>[8x]MHHHHHHGENLYFQGSMLTIVQEALTFDDVLLLPAYSTVLPKDVSLKTRLTRGIYLNIPLVSAAMDTVTESRMAIAMAQNGGIGILHKNMDIAAQAAEVRRVKKFEAGKAESYPNSCKDDLGRLRVGAAVGTGADTPSRV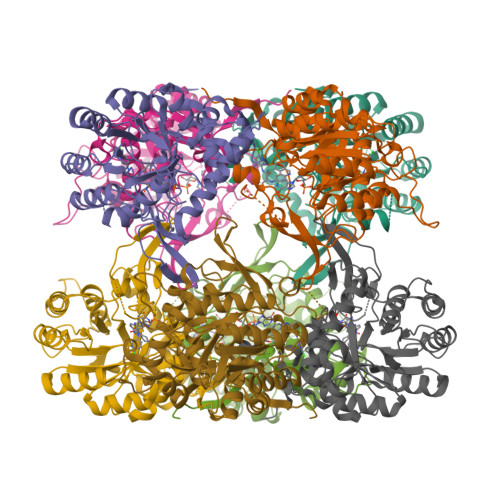EALVEAGVDVIVVDTAHGHSAGVIERVRWVKQNFPQVQVIGGNIATGDAALALLDAGADAVKVGIGPGSICTTRIVAGIGMPQISAIDSVASALKDQIPLIADGGIRFSGDMAKAIGAGASTIMVGSLLAGTEEAPGEVEFFQGRYYKAYRGMGSLGAMAGATGSADRYFQDSKAGAEKLVPEGIEGRVPYKGPMGNIVHQMMGGLRSSMGYTGSAVIEDLRQNAKFVKITSAGMSESHVHDVTITKEAPNYRVG5-(3,6-dihydro-2~{H}-pyran-4-yl)-2-methoxy-~{N}-[5-[3-(4-propan-2-ylpiperazin-1-yl)prop-1-ynyl]pyridin-3-yl]pyridine-3-sulfonamide | C26 H33 N5 O4 S | 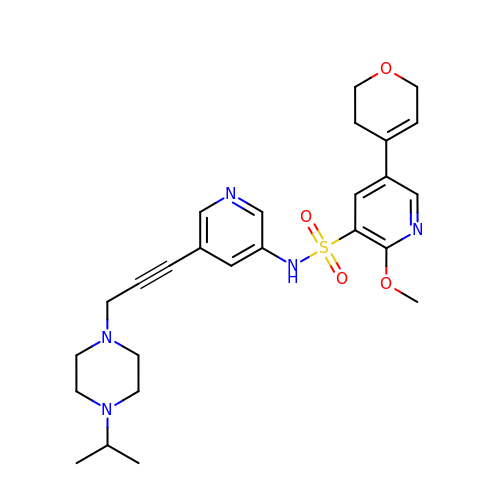WSRDHUWKQAFXNI-UHFFFAOYSA-N>[2x]MSSERTFIAVKPDGVQRGLVGEIIARFERKGYKLVALKILQPTTEQAQG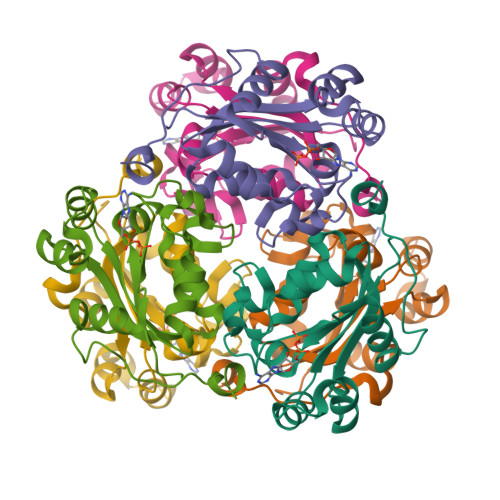HYKDLCSKPFFPALVKYFSSGPIVCMVWEGKNVVKSGRVLLGATNPADSQPGTIRGDFAVDVGRNVCHGSDSVESAEREIAFWFKADEIASWTSHSVSQIYE>[10x]MIQSQINRNIRLDLADAILLSKAKKDLSFAEIADG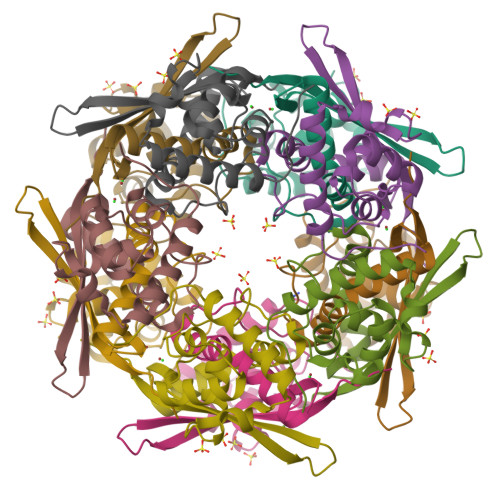TGLAEAFVTAALLGQQALPADAARLVGAKLDLDEDSILLLQMIPLRGCIDDRIPTDPTMYRFYEMLQVYGTTLKALVHEKFGDGIIGAINFKLDVKKVADPEGGERAVITLDGKYLPTKPF Here we show that a dominant member of the human microbiota, Bacteroides ovatus, contains a GH115 enzyme, BoAgu115A, which displays glucuronoxylan α-(4-O-methyl)-glucuronidase activity. The enzyme is significantly more active against substrates in which the xylose decorated with GlcA/MeGlcA is flanked by one or more xylose residues. The crystal structure of BoAgu115A revealed a four-domain protein in which the active site, comprising a pocket that abuts a cleft-like structure, is housed in the second domain that adopts a TIM barrel-fold. The third domain, a five-helical bundle, and the C-terminal β-sandwich domain make inter-chain contacts leading to protein dimerization.

The crystal structure of the native BoAgu115A was solved by extending the phase information from an initial selenomethionine SAD at 3.0 Å to a native resolution of 2.65 Å, whereas the ligand structure of the enzyme was determined by molecular replacement at a resolution of 2.14 Å. The center of the cleft, which may accommodate the xylan backbone, abuts onto a deep pocket that likely comprises the active site. This hypothesis was confirmed when BoAgu115A was co-crystallized with GlcA, which revealed electron density for the uronic acid in the proposed active site pocket. The sugar was found to be in its ring open conformation, which is highly unusual for hexaose aldehyde sugars. It is possible that the specific interactions between the uronic acid and the enzyme encourage GlcA to adopt an open chain conformation after glycosidic bond cleavage. The direct interactions between GlcA and the enzyme are as follows: O3 makes a polar contact with Nϵ-1 of Trp-249. O6A and O6B of the uronic acid carboxylate form polar contacts with the OH of Tyr-420 and Nϵ-2 of His-422, respectively, the endocyclic oxygen interacts with the N of Val-426, and O1 makes a hydrogen bond with Asp-206. O4 is pointing into a hydrophobic open channel, comprising the side chains of Phe-203, Met-248, and Trp-245, which likely make apolar contacts with the methyl group of MeGlcA. Unlike the vast majority of glycoside hydrolases, the active site of BoAgu115A does not make typical parallel stacking interactions between the planar faces of aromatic residues and the sugar ring, although edge on edge apolar interactions between the sugar and two aromatic residues, Trp-249 and Tyr-420, and the aliphatic side chain of Val-426 were evident. Indeed, in the BoAgu115A-GlcA structure the loop that contains Asp-332 (Met-327 to Asn-346) was too disordered to be modeled, whereas Glu-375 could not be built past the β-carbon. Furthermore, the loop also plays a role in stabilizing residues in the putative xylan binding cleft, notably Lys-374 and Glu-782, whose side chains are disordered in the GlcA bound structure where the loop is too flexible to be modeled.

>[2x]MINNKLLNIETMKKLFLFFYLSVVSIAAFAAEQFVIFTPAGNHFPLVANGVPCPIYIDSSEDKGVMIAAGNLQQDILQVCGKKPELLTSTSSKRCIIAGTYGTPFIKKLMSAGKIDKKELDGKNEKYILQVIANPCEGIDEAVVIIGSDRRGTIYGIYELSEQMGVSPWYWWADVPVMKQANVYIKPGQYSDGEPAVTYRGIFLNDEAPCLTRWVKHTYGTNYGDHRFYARVCELILRLKGNFLWPAMWSWAFYADDPQNSKTASEMGVIIGTSHHEPMARNHQEWSRKRKEYGAWDYTTNQKVIDQFFREGIERMQGTEDIVTIGMRGDGDAAMSKSTNVKLLENVVKNQRKIIEEVTKRPAKETPQVWALYKEVLDYYDKGMRVPDDVIMLLCDDNWGNVCRLPNAKERKHPGGWGMYYHVDYVGAPRNSKWLNVTPIQNMWEQLQLTYDYGVEKLWILNVGDLKPMEYPITLFMDMAWNPKQFNVSNLLDHPRRFCAQQFGEDQADEAMRILNLYSKYNGRVTGEMLDRNTYNLETGEWKQVSDEYLKLEAEALRQYISLKPEYKDAYKQLILFPVQAMANLYEMYYAQAMNHKLYKENNPQANEWADKVEQAFARDKALSDDYNNIMSGGKWKNMMIQKHIGYTSWNDNFPADTLPKIYRIENPEKAVGGYVFTGQDGYIAIEAEHYYSAKAAPDTEWTVIPYMGRTLSGMALMPYTQPTDGASISYKIKLPKGIDKVTVHVIVKSTLAFHDRKGHEYSIGFEGGKDQTINFNHNLNELPENVYSIYYPTVARRIVEKKAKLNVPNTSDGMQTITFKPLDPGIVLEKLVVDYGGYKKSYLFMNESKSKRESR ethylboronic acid | C2 H7 B O2 | 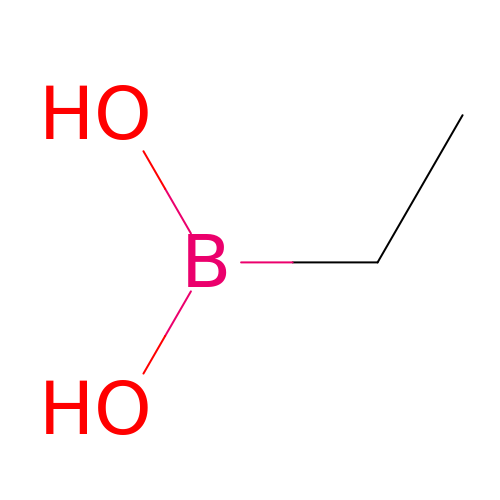PAVZHTXVORCEHP-UHFFFAOYSA-N>[2x]MYRPKDHGWVEVIVGPMYSGKSEELIRRIRRAKIAKQKIQVFKPEIDNRYSKEDVVSHMGEKEQAVA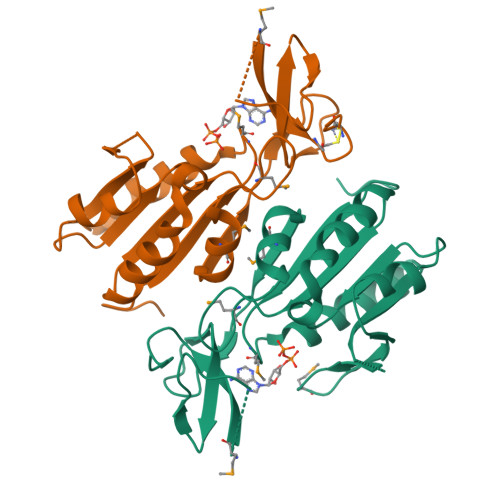IKNSREILKYFEEDTEVIAIDEVQFFDDEIVEIVNKIAESGRRVICAGLDMDFRGKPFGPIPELMAIAEFVDKIQAICVVCGNPATRTQRLINGKPAFYDDPVVLIGAMESYEARCRKCHVVPQ> MDIFREIASSMKGENVFISPPSISSVLTILYYGANGSTAEQLSKYVEKEADKNKDDISFKSMNKVYGRYSAVFKDSFLRKIGDNFQTVDFTDCRTVDAINKCVDIFTEGKINPLLDEPLSPDTCLLAISAVYFKAKWLMPFEKEFTSDYPFYVSPTEMVDVSMMSMYGEAFNHASVKESFGNFSIIELPYVGDTSMVVILPDNIDGLESIEQNLTDT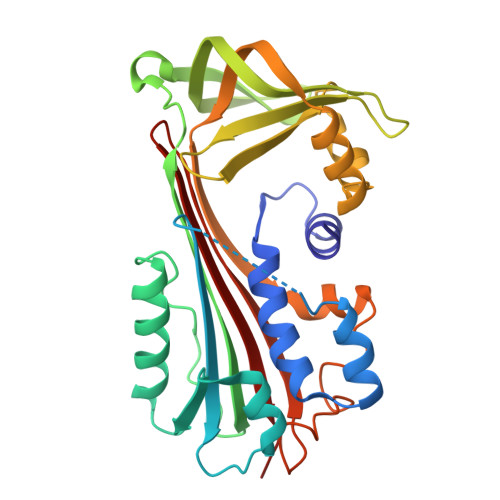NFKKWCDSMDAMFIDVHIPKFKVTGSYNLVDALVKLGLTEVFGSTGDYSNMCNSDVSVDAMIHKTYIDVNEEYTEAAAATCALVADCA3-(carbamoylamino)-5-phenylthiophene-2-carboxamide | C12 H11 N3 O2 S | 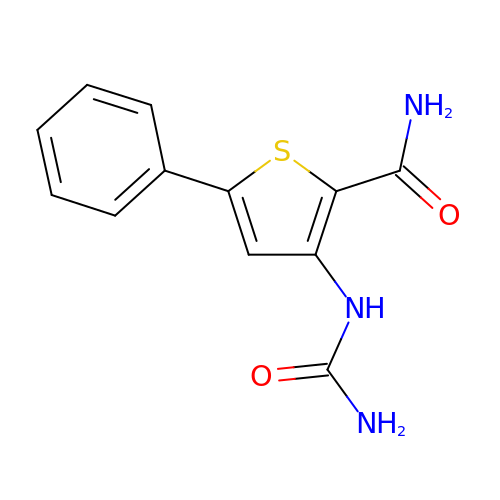HKWYRLYHYBFHLL-UHFFFAOYSA-N> MCIEFAFKKAGIPIVRNFLHSTEGVIYGLPQRVQRNLAINYTVKQYKEGKAVSAKTIK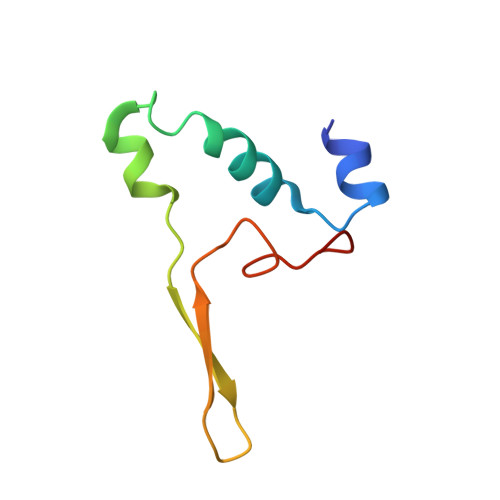TLQEAFPSKGDTK> MMNAKSLLRWAGALVAVAAVTVFGLDARGTTKPLPGSTGEQRADLVEIGVMAKFGNLELPKVTFPHDRHSEAVAKVAAPGKECATCHKNDDKGKMSLKFMRLEDTTAADLKNIYHANCIGCHTEQAKAGKKTGPQDGECRSCHNPKPMASSWKQIGLDKSLHFRHVAAKAIAPVNDPQKNCGACHHVYDEAAKKLSWVKNKEDSCRACHGDARVEKKPSLREAAHTQCITCHRSVAAAPAKADSGPVSCAGCHDPAMQAKFKVVRDVPRLERGQPDAAMVLPVVGPGAKDTPKGMKGAMKPVAFNHKVHEAASNTCRACHHVKIDNCTTCHTLEGVKDGNFVQIE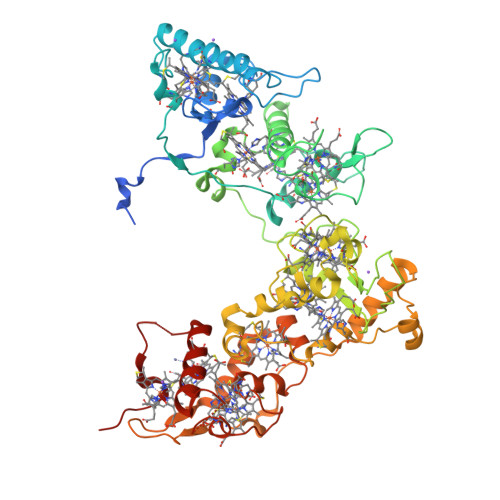KAMHQPDSMKSCVGCHNQKVQAPACAGCHGFMKTGAKPQPEAACGVCHADPVGMDAKTVADGGLLKATKEQRADVAAATLAARRTTKGTLPADDIPEFVTIGVLSDKYEPSKLPHRKIVNTLMAAIGDDKLAGTFHTDKATVCAGCHHNSPASKTPPKCASCHGQPFDAAKGDRPGLKAAYHQQCMGCHNRMKLEKPADTACAECHKERAK>DSTTPGYTVVKNDWKKAVKQLQDGLKNKTISTIKVSFNGNSVGEVTPASSGAKKADRDAAAEKLYNLVNTQLDKLGDGDYVDFEVTYNLATQIITKAEAEAVLTKLQQYNDKVLINSATDTVKGMVSDTQVDSKNVAANPLKVSDMYTIPSAITGSDDSGYSIAKPTEKTTSLLYGTVGDATAGKAITVDTASNEAFAGNGKVIDYNKSFKATVQGDGTVKTSGVVLKDASDMAATGTIKVRVTSAKEESIDVDSSSYISAENLAKKYVFNPKEVSEAYNAIVALQNDGIESDLVQLVNGKYQVIFYPEGKRLETKS[2x];>[2x]ADIIADADSPAKITIKANKLKDLKDYVDDLKTYNNTYSNVVTVAGEDRIETAIELSSKYYNSDDKNAITDDAVNNIVLVGSTSIVDGLVASPLASEKTAPLLLTSKDKLDSSVKSEIKRVMNLKSDTGINTSKKVYLAGGVNSISKDVENELKNMGLKVTRLSGEDRYETSLAIADEIGLDNDKAFVVGGTGLADAMSIAPVASQLKDGDATPIVVVDGKAKEISDDAKSFLGTSDVDIIGGKNSVSKEI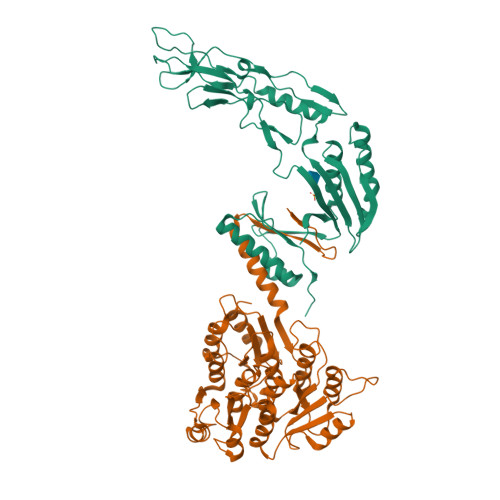EESIDSATGKTPDRISGDDRQATNAEVLKEDDYFKDGEVVNYFVAKDGSTKEDQLVDALAAAPIAGRFKESPAPIILATDTLSSDQNVAVSKAVPKDGGTNLVQVGKGIASSVINKMKDLLDM>GHMVPQTGRAARATRESGRQTRDALFTAATELFLEHGEGVPITQICAAAGAHPNQVTYYYGSKERLFVEVACAAVLRAGKRAEDDAATAETVGDYTEKLVGSLLGPGAPSVELFTSAMLMTGRRSELRDLITDTLRTLHSSGEVALIRTLMRTGWQLRAGIDVESKAFWSAIFGLV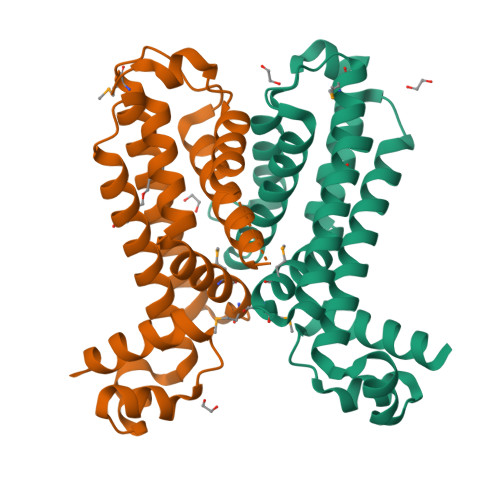IQKTATGESFGYSLEEAVAVIFANLQIPETVRNTSIDGS[2x]>[2x]SNAMVRVGTIAGPETQLMEVAKQVALNRYGLHVNIITFSDYNTPNEALADGSVDANMFQHLPYLKAQIEMRGYKIVSIGKTFVY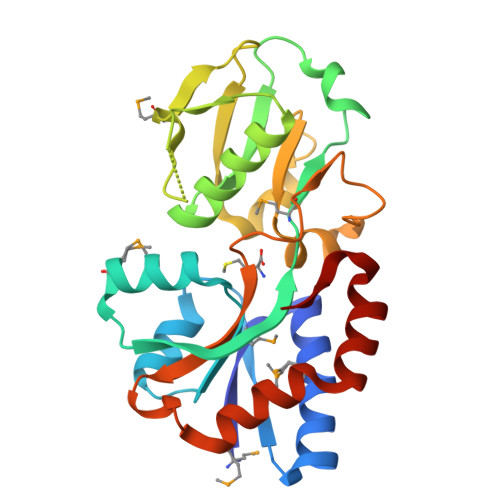PMGLYSKKITALTQLKTGAKIAVPSDPSNEARALLLLEKAQLIQLKTHVTINATPMDIASNPKKLKIVELDAAQLSRSLGDVDLAAINTNYAIPAGLSPSRDALLTEGPNSPYANVVAVREDDKNDPRLKQLVSALHSPAVLSAAKKIFGDGAIPA>MKHLLKAGALVALACIVTLTAGAQAHAAKRINIRLAHPMAPGNNVTVGYEKFKELVAEKSNGRVRIQLFGNCMLGSDRVTMEAAQRGTLEMASSSSPNMANFSKQWMVFDLPYITSPEHQQKLYKAIDDGELGKKLDEIAASIGLKPIMYSEYGYRNFVTTKKPIKTADDLKNLKVRTTDSPIEVAVAAALGMAPTPISWGETYTALQQGTVDGEGNTFSLLNDAKHTEVLKYAIDSAHNYSMHLLMMNKAYYDSLPANVQQILTEAGREALTYQRSITSELEKKAEDAFIEQGITVTRLSPEERAKLVERTRPVWDKFKDDIPAELIKLVQETQQ[2x]

O. alaskensis employs a tripartite ATP-independent periplasmic (TRAP) transporter (OaIsePQM) to import isethionate, which relies on the substrate-binding protein (OaIseP) to scavenge isethionate and deliver it to the membrane transporter component (OaIseQM) for import into the cell. Like the ATP-binding cassette importers, TRAP transporters utilise a high-affinity substrate-binding protein (P-subunit) that binds the organic acid and delivers it to the membrane-spanning transporter subunits (Q and M) for uptake. The structure of TRAP substrate-binding proteins comprises two globular lobe-like domains connected by a variable hinge region, which is formed by two β-strands and a unique extended α-helix. Substrates bind within the cleft between the two domains, which close around the bound substrate via a hinge-bending conformational change often described as a ‘Venus flytrap’ mechanism.

To define the molecular details of substrate-binding, we determined the isethionate-bound structure of OaIseP. OaIseP purified in 5 mM isethionate produced crystals that diffracted to 1.25 Å. The asymmetric unit for isethionate-bound OaIseP contained two monomers that are bridged by water molecules, where domains I and II of each monomer interact with domains II and I of the opposing monomer. We used Proteins, Interfaces, Structures and Assemblies (PISA) to assess the nature of the interface between chains A and B, calculating the size of the buried area to be 624 Å2, with a Complexation Significance Score of 0, which suggested that the formation of this assembly was not likely. Isethionate is bound in the cleft between domain I and domain II, with a closer examination of the isethionate-binding site revealing several key contacts made by OaIseP. The sulfonate moiety of isethionate forms salt bridges with Arg156 and Arg177, as well as forming hydrogen bonds with Ser95, Asn98, Tyr153, and Asn217. At the opposing end of isethionate, hydrogen bonds are formed with Asn77 and His244 via the terminal hydroxyl group. No water molecules directly contact isethionate, and the binding site is lined with Pro38, Met39 and Leu221, with Trp200 occupying the bottom of the site, providing a large hydrophobic surface for the hydrocarbon backbone of isethionate. Aligning the open ligand-free and closed isethionate-bound structures gives an r.m.s.d. of 2.7 Å over all 308 pairs of α-carbons. The conformational change primarily involves bending of the hinge region within the spanning α-helix and nearby β-strands that connect the two domains.>[2x]MSSMEGKKVPQVTFRTRQGDKWVDVTTSELFDNKTVIVFSLPGAFTPTCSSSHLPRYNELAPVFKKYGVDDILVVSVNDTFVMNAWKEDEKSENISFI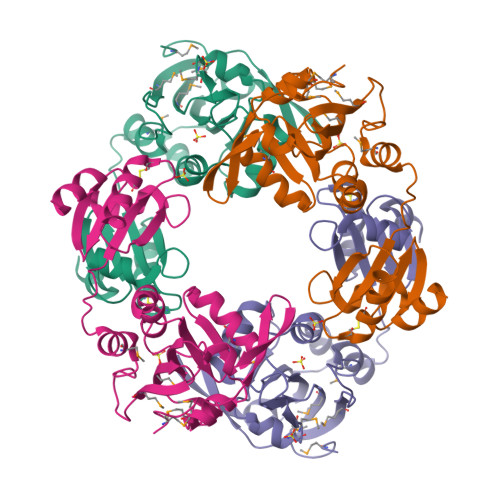PDGNGEFTEGMGMLVGKEDLGFGKRSWRYSMLVKNGVVEKMFIEPNEPGDPFKVSDADTMLKYLAPQHQVQESISIFTKPGCPFCAKAKQLLHDKGLSFEEIILGHDATIVSVRAVSGRTTVPQVFIGGKHIGGSDDLEKYFA> ISHMSINIRDPLIVSRVVGDVLDPFNRSITLKVTYGQREVTNGLDLRPSQVQNKPRVE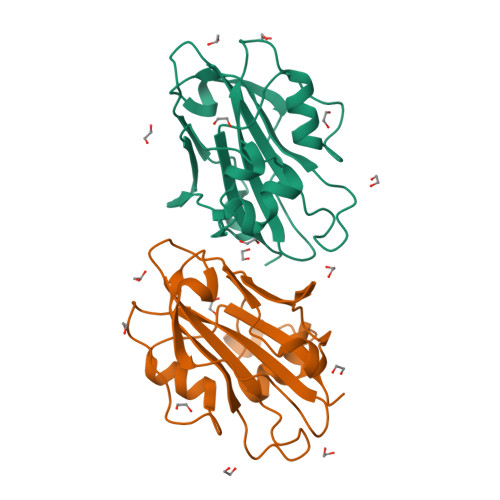IGGEDLRNFYTLVMVDPDVPSPSNPHLREYLHWLVTDIPATTGTTFGNEIVSYENPSPTAGIHRVVFILFRQLGRQTVYAPGWRQNFNTREFAEIYNLGLPVAAVFYNSQRES> GSIMRDINKLEEQNPDIVSEKKPATEVDPTHFEKRFLKRIRDLGEGHFGKVELCRYDPEGDNTGEQVAVKSLKPESGGNHIADLKKEIEILRNLYHENIVKYKGICTEDGGNGIKLIMEFLPSGSLKEYLPKNKNKINLKQQLKYAVQICKGMDYLGSRQYVHRDLAARNVLVESEHQVKIGDFGLTKAIETDKEYYTVKDDRDSPVFWYAPECLMQSKFYIASDVWSFGVTLHELLTYCDSDSSPMALFLKMIGPTHGQMTVTRLVNTLKEGKRLPCPPNCPDEVYQLMR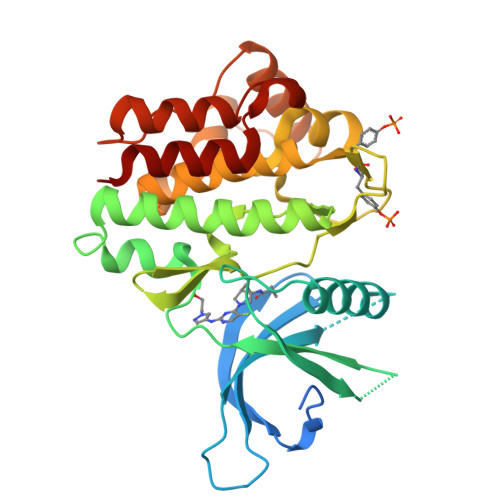KCWEFQPSNRTSFQNLIEGFEALLK> HLIPAQQRTVEHLDAMQWINGDGYLHNVFVRWFNGDVIRPKTWFWQDVKTRKILGWRCDVSENIDSIRLSFMDVVTRYGIPEDFHITIDNTRGAANKWLTGGAPNRYRFKVKEDDPKGLFLLMGAKMHWTSVVAGKGW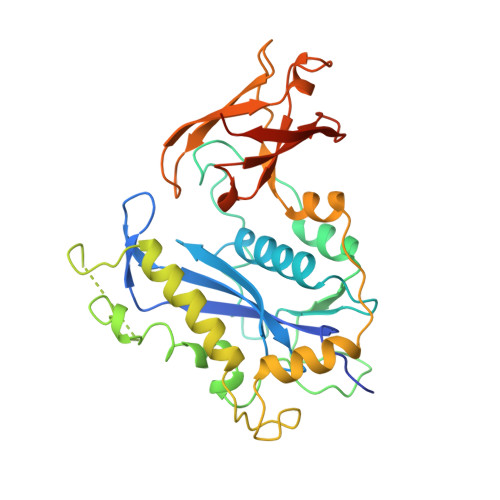GQAKPVERAFGVGGLEEYVDKHPALAGAYTGPNPQAKPDNYGDRAVDAELFLKTLAEGVAMFNARTGRETEMCGGKLSFDDVFEREYARTIVRKPTEEQKRMLLLPAEAVNVSRKGEFTLKVGGSLKGAKNVYYNMALMNAGVKKVVVRFDPQQLHSTVYCYTLDGRFICEAECLAPVAFNDAAAGREY> NTKYNKEFLLYLAGFVDSDGSIIAQIKPNQSVKFKHRLQLTFDVTQKTQRRWFLDKLVDEIGVGYVADSGSVSKYRLSEIKPLHNFLTQLQPFLKLKQKQANLVLKIIEQLPSAKESPDKFLEVCTWVDQIAALNDSKTRKTTSETVRAVLDSL;> NTKYNKEFLLYLAGFVDGDGSIIAQIKPNQSGKFKHKLSLTFKVTQKTQRRWFLDKLVDEIGVGYVYDSGSVSNYYLSEIKPLHNFLTQLQPFLKLKQKQANLVLKIIEQLPSAKESPDKFLEVCTWVDQVAALNDSKTRKTTSETVRAVLDSL

I-CreI is a homodimeric member of LHEs family, which recognizes and cleaves a 22 bp pseudo-palindromic target (5′- CAAAACGTCGTGAGACAGTTTG -3′). Each I-CreI monomer binds its own DNA target region generating the catalytic centre at the dimer interface. This region contains two catalytic aspartic acids (D20, one per each monomer). The aspartic side chains participate in the cleavage of the DNA strands along the minor groove, resulting in the hydrolysis of specific phosphodiester bonds upon the coordination of three divalent metal ions.

To broaden our analysis, we also studied the I-CreI heterodimeric variant I-CreI_3115 (Y33G/Q38K/Q44K/R68Y/R70S/D75N/I77Y/I132V-G19S/Y33V/Q38R/S40Q/Q44D/R68A/R70S/D75K/I77R). This mutant was generated using the methodology previously described, and is able to recognize and cleave the human HBB (Haemoglobin beta subunit) gene (I-CreI_3115_target, Fig. 1c upper sequence) whose mutations cause sickle cell anaemia. To understand the molecular mechanism that inhibits cleavage when a G is at −4 position flanked by a pyrimidine at position −5, we solved the crystal structures of the cleavable and the corresponding non-cleavable variant targets in the presence of catalytic (Mg2+) and non-catalytic (Ca2+) cations. As expected from in vitro cleavage experiments, the comparison of the crystal structures of the I-CreI variants in complex with its cleavable and non-cleavable target DNAs in favourable catalytic conditions (2 mM Mg2+), showed the hydrolysed phosphodiesters in the cleavable targets while the non-cleavable targets displayed the intact phosphodiester bonds. We observed that the structures of the variants in complex with the cleavable targets showed the presence of the 3 reported catalytic ions, while the structures in complex with the non-cleavable targets indicated the presence of just 2 catalytic ions, with the central metal position occupied by a water molecule. On the other hand, when the two enzyme variants were simulated bound to the I-CreI_D75N_target and I-CreI_3115_target DNA sequences, the helical parameters of A +1 were similar to those found in the ideal B-DNA conformation, with minor fluctuations typical of atomic thermal motions.BrlR, a member of the MerR family of multidrug efflux pump activators, consists of a structurally conserved N-terminal DNA-binding domain and a C-terminal GyrI-like binding domain. BrlR mediates the antibiotic resistance of P. aeruginosa by activating the expression of multidrug efflux pumps and repressing PhoPQ activation. The monomer can be divided into three domains: the N-terminal DNA-binding domain (residues 1–75), which adopts a winged helix-turn-helix fold; the long central α-helical linker (residues 76–119), which connects two terminal domains; and the C-terminal multidrug-binding domain (residues 120–270). Our most striking finding is that BrlR is not only a pyocyanin receptor but it is also a dual receptor that is responsive to both c-di-GMP and pyocyanin.

The structure of the BrlR–c-di-GMP complex belongs to space group I4. Each asymmetric unit contains two BrlR monomers and four c-di-GMP molecules. The monomer of the BrlR–c-di-GMP complex contains two c-di-GMP binding sites in different regions on the DNA-binding domain. The DNA-binding domain contains two separate c-di-GMP-binding sites, and shares a mutually intercalated c-di-GMP dimer in a stacking conformation with a crystallographic symmetry related binding site. Thus, the overall structure reveals a receptor–ligand complex with a 1:2 stoichiometry. The structure shows that the 2′-hydroxyl group of the c-di-GMP molecule in each site points toward the solvent and is not involved in the binding to BrlR. Crystallographic symmetry analysis indicates that the BrlR-c-di-GMP complex also forms a stable homotetramer, which is made up of two dimers as the final model of apo-BrlR (AA′ and BB′). Overall, the c-di-GMP-bound BrlR has a larger positively charged surface than apo-BrlR on the DNA-binding domain, and the simultaneous occupation of the two c-di-GMP binding sites twists and bends the DNA-binding domain and the coiled-coil linker. The recognition helix (α2) of the HTH motif is 1.2 Å shorter (Cα(H20)–Cα(H20′)) in the BrlR-c-di-GMP complex than that in apo-BrlR, which could help BrlR approach DNA.

>[2x]GSMLTIGQLARIFEISTKTLRHYDAIGLFVPARTGSDNGYRYYQPEQIEQLSRILALRRLDVPLEAIDRLKRDGALDDPQRLRHFLQRHQHTLREEISARQRLLAELDRTLATLAHWRIRNMHARIVERPAFSVVGMEYFGSAPGDTIGQLWERFIPREHEIAGKHDPEVSYGICAQQPNGEFHYVAGFEVQEGWPVPEGMVRFQVPAQKYAVFTHKGTAPQIAESFQAIYSHLLAERGLEPKAGVDFEYYDQRFRGPLDPNSQVDLYIPIY3-(4-oxo-3,4-dihydroquinazolin-2-yl)-N-[(1S)-1-phenylethyl]propanamide | C19 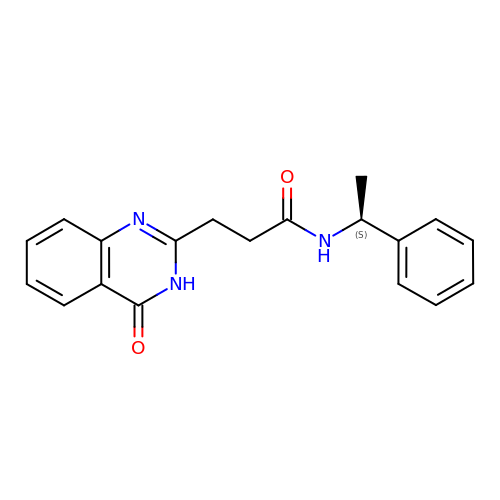H19 N3 O2 | QIHBWVVVRYYYRO-ZDUSSCGKSA-N>ASMTGGQQMGRDQAGITGTWYNQLGSTFIVTAGADGALTGTYVTARGNAESRYVLTGRYDSAPATAGSGTALGWTVAWKNNYRNAHSATTWSGQYVGGAEARINTQWLLTSGTTEANAWRSTLVGHDT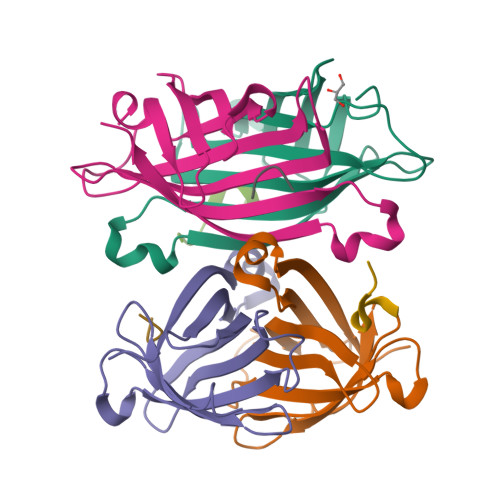FTKVQPSAASIDAAKKAGVNNGNPLDAVQQ[4x];>[4x]XPWSHPQFEK> ANNLPDTQSSGPAHSKETPALTAVETGATNPLVPSDTVQTRHVIQKRTRSESTVESFFARGACVAIIEVDNDAPTKRASKLFSVWKITYKDTVQLRRKLEFFTYSRFDMEFTFVVTSNYTDANNGHALNQVYQIMYIPPGAPIPGKWNDYTWQTSSNPSVFYTYGAPPARISVPYVGIANAYSHFYDGFAKVPLAGQASTEGDSLYGAASLNDFGSLAVRVVNDHNPTKLTSKIRVYMKPKHVRVWCPRPPRAVPYYGPGVDYKDGLAPLPGKGLTTY;> SVRVMQLTLGNSTITTQEAANSVVAYGRWPEYIKDSEANPVDQPTEPDVAACRFYTLDTVTWRKESRGWWWKLPDALKDMGLFGQNMFYHYLGRAGYTVHVQCNASKFHQGALGVFAVPEMCLAGDSTTHMFTKYENANPGEKGGEFKGSFTLDTNATNPARNFCPVDYLFGSGVLAGNAFVYPHQIINLRTNNCATLVLPYVNSLSIDSMTKHNNWGIAILPLAPLDFATESSTEIPITLTIAPMCCEFNGLRNITVPRTQ;> GLPVLNTPGSNQYLTADNYQSPCAIPEFDVTPPIDIPGEVRNMMELAEIDTMIPLNLTNQRKNTMDMYRVELNDAAHSDTPILCLSLSPASDPRLAHTMLGEILNYYTHWAGSLKFTFLFCGSMMATGKLLVSYAPPGAEAPKSRKEAMLGTHVIWDIGLQSSCTMVVPWISNTTYRQTINDSFTEGGYISMFYQTRVVVPLSTPRKMDILGFVSACNDFSVRLLRDTTHISQEA;> GAQVSSQKVGAHENSNRAYGGSTINYTTINYYRDSASNAASKQDFAQDPSKFTEPIKDVLIKTAPTLN;> VVQAPTQVPGFLGDSVTLPCYLQVPNMEVTHVSQLTWARHGESGSMAVFHQTQGPSYSESKRLEFVAARLGAELRDASLRMFGLRVEDEGSYTCLFVTFPQGSRSVDIWLRVLAKPQNTAEVQKVQLTGEPVPMARCVSTGGRPPAQITWHSDLGGMPQTSQVPGFLSG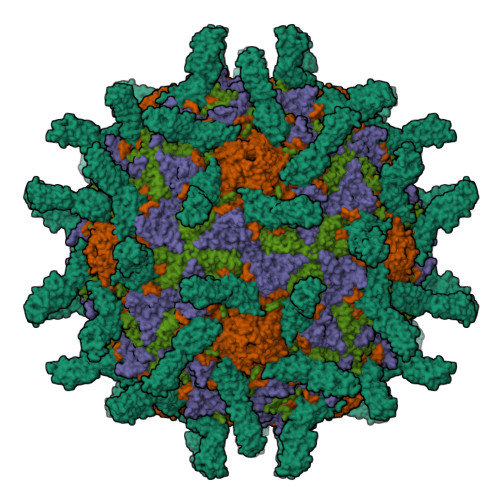TVTVTSLWILVPSSQVDGKQVTCKVEHESFEKPQLLTVSLTVYY> MALKALILNT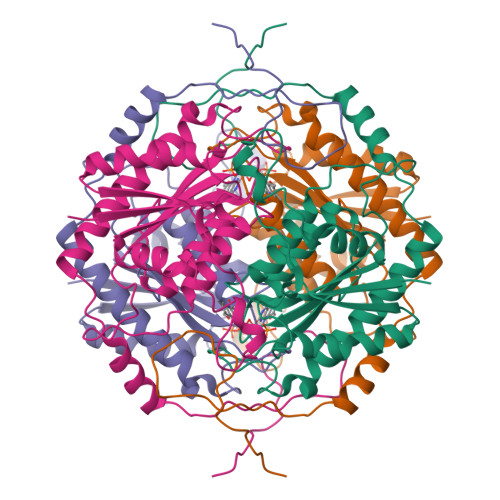TLRRSPSRSQTQGLIDKAVPLYEKEGIETEVVRVIDHDIEQEYWDDYDDWNAGEKARREDEWPWLLEKIREADILVIATPITLNMCTSAAHVILEKLNLMDELNGDTKQFPLYNKVAGLLMCGNEDGAHHVAGTVLNNLGRLGYSVPPNAAAYWLGPAGTGPGYIEGKGDRHFHTNKLIRFMVANTSHLARMLQETPYTTDLEACAQAAREESDDVFAIRVNVNTPAIRYKRFQKLGEVKVEESQLG> G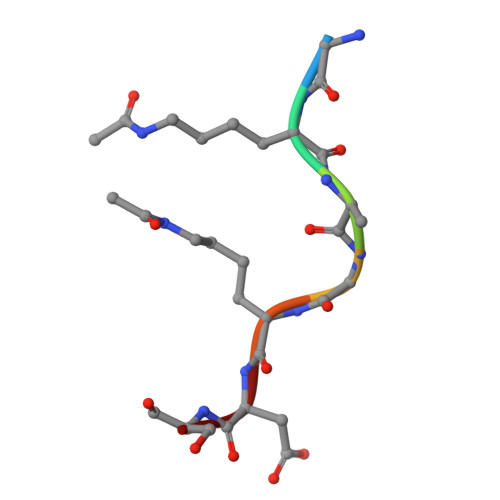KAGKDS> MDL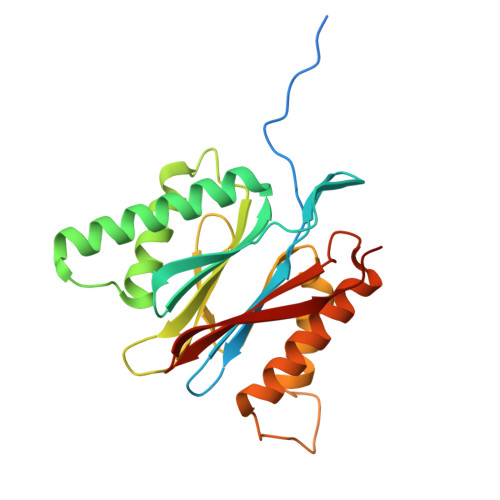ILYNDNLTEKKTEKENVIEHGRGFKRWYPYIDNGGTVIGLTGKDYVILAADTRLSLSYSIYTRFCPKISKLTDKCIIGSSGMQSDIKTLHSLLQKKIQLFVLEHSHYPDIHVIDRLLCVILYSRRFFPYYAFNILAGVDENNKGVLYNYDSVGSYCEATHSCVGSGSQLILPILDNRVEQKNQLIKNTNFNLGDDINFVKDAITSATERDIYTGDKTLIYVIDKMGINVNTLDLKQD>MGMKSATMSATHALRDKWFVSFLPLLTADMVNTDYKGNWQLAAQERTQKLDWITSVEELWSTMNSLPKVHQLGMGSTLIFARNNKEPPSYEAYPNGSRIMINLLKPPTTDAGLELVLAVVMGETAAEKASDGKPVCDVLRIAARPSREHSEQIRVEVWLSDSTRSHAVAEFLAEAMRAKGLAANSYNIAEASFDAAA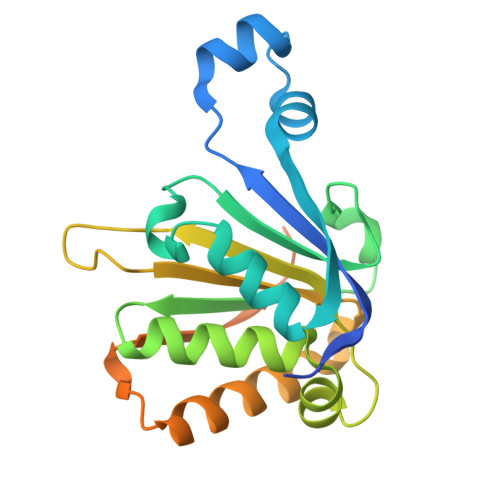PGKDKKVLAASTMPSPSSPPMVKDAAALEHHHHHH[2x]>[2x]GPWADIMQGPSESFVDFANRLIKAVEGSDLPPSARAPV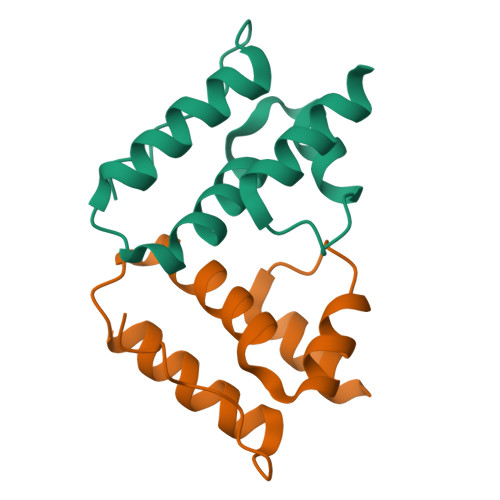IIDCFRQKSQPDIQQLIRTAPSTLTTPGEIIKYVLDRQKTAPLTDQGIA>MLVVGSELQSDAQQLSAEAPRHGELQYLRQVEHILRCGFKKEDRTGTGTLSVFGMQARYSLRDEFPLLTTKRVFWKGVLEELLWFIKGSTNAKELSSKGVRIWDANGSRDFLDSLGFSARQEGDLGPVYGFQWRHFGAEYKDMDSDYSGQGVDQLQKVIDTIKTNPDDRRIIMCAWNPKDLPLMALPPCHALCQFYVVNGELSCQLYQRSGDMGLGVPFNIASYALLTYMIAHITGLQPGDFVHTLGDA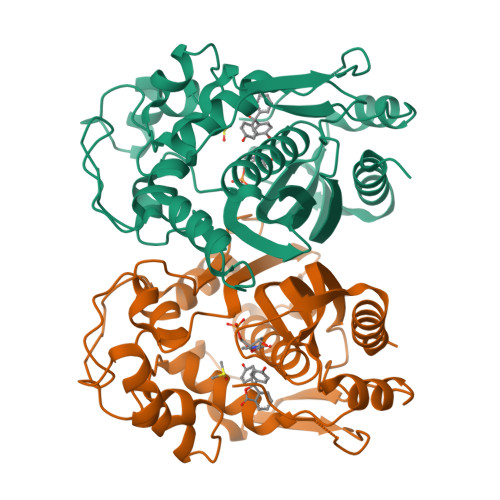HIYLNHIEPLKIQLQREPRPFPKLKILRKVETIDDFKVEDFQIEGYNPHPTIKMEMAV[2x]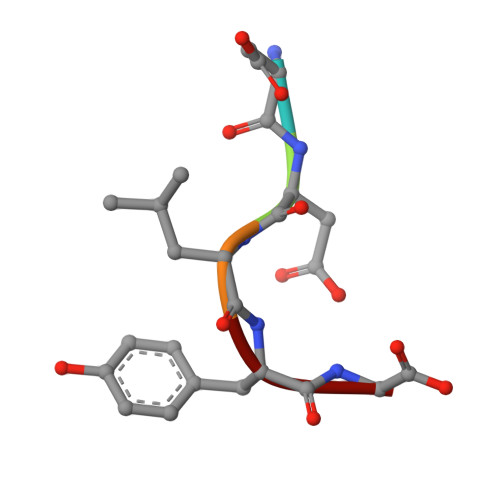> DDLYG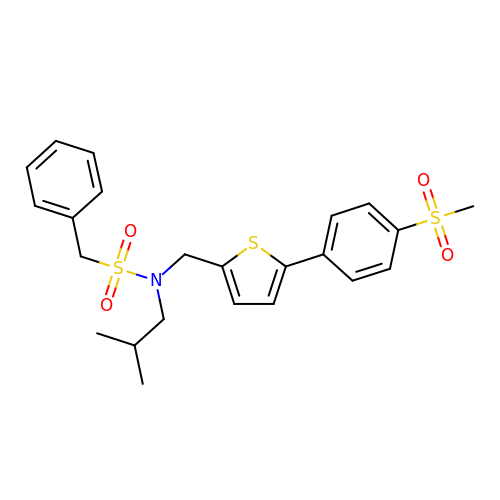N-(2-methylpropyl)-N-({5-[4-(methylsulfonyl)phenyl]thiophen-2-yl}methyl)-1-phenylmethanesulfonamide | C23 H27 N O4 S3 | RXMHSSANSKRGOG-UHFFFAOYSA-N>MALAKIVFASMTGNTEEIADIVADKLRDLGLDVDVDECTTVDASDFLEADIAIVATYTYGDGELPDEMMDFYEDLADLNLNGKIYGVVGSGDTFYDEFCKAVDDFDRVFVSTGAEKGSECVKVDLSAEEEDIERLEQFAEELAAK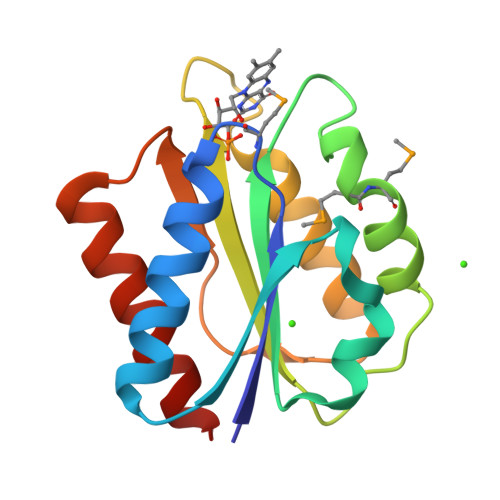VGA[2x]The next step is the formation of the indole moiety, which is catalyzed by indole-3-glycerol phosphate synthase (IGPS; the product of trpC). This reaction comprises a ring closure of the substrate 1-(o-carboxyphenylamino)-1-deoxyribulose-5-phosphate (CdRP) into the product indole-3-glycerol phosphate (IGP). The IGPS structure has a canonical (βα)8-barrel fold with an additional N-terminal helical extension comprising two α-helices, α0 and α00, of which α0 forms a lid over the active site. In this work, we have probed the structure and mechanism of IGPS from P. aeruginosa, because it has the highest reported turnover number of all IGPS enzymes characterized to date.

The PaIGPS–rCdRP complex crystallized in space group P21212 in a large unit cell containing eight enzyme molecules per asymmetric unit. The substrate analog, rCdRP, is bound in the active site of the seven more ordered chains. rCdRP is enclosed in the active site by the helix α0 and βα-loops 1, 2, and 6. The suggested catalytic residues (Lys123, Glu172, Lys63, and Glu61) adopt similar conformations and identical interactions with the ligand rCdRP as in the SsIGPS structure. In chain B, the same conformation of rCdRP does not fit the electron density, and the ligand instead adopts a conformation where the C2' hydroxyl is shifted 2.2 Å toward the general acid Lys123. The observed movements in the C1'–C2' region in some chains are possibly coupled to the position of the guanidinium group of Arg196 on loop 6, which adopts an “inward” conformation and interacts with both the ligand's carboxylate and phosphate group in chains B, F, G, and H. Chain G lacks density for rCdRP in the active site. The helix adopts an open conformation in chain G, where—through domain swapping—it covers the active site of a symmetry-related molecule. Moreover, the disorder of these three regions reflect their innate flexibility in the apo state and suggest an induced fit mechanism of substrate binding. However, in PaIGPS, there is a phenylalanine on active-site βα-loop 6 (Phe201), 4 Å away from the anthranilate of rCdRP, whereas in EcIGPS the corresponding residue is a leucine. PaIGPS has the highest reported turnover, and from structure-guided mutagenesis we find that an active-site phenylalanine is responsible for its high activity compared with other IGPS enzymes, possibly by guiding the rate-limiting condensation step.

>[7x]MSVPTVLQKILARKAEEVAERRARVNLAEVERLARSADAPRGFANALLERAKRKEPAVIAEIKKASPSKGVLREHFVPAEIARSYEAGGAACLSVLTDVDFFQGADAYLKEARAACALPVIRKDFMIDPYQIVEARAIGADCILLIVSALDDVLMAELAATAKSVGLDVLVEVHDGTELERALKTLDTPLVGINNRNLHTFEVSLETTLDLLPEIPRDRLVVTESGILNRADVELMEVSEVYAFLVGEAFMRADDPGLELKRLFFQERGAVVLGADPDTSGHHHHHH;> XXXXXXXXXXXXXXVNLAEVERLARSADAPRGFANALLERAKRKEPAVIAEIKKASPSKGVLREHFVPAEIARSYEAGGAACLSVLTDVDFFQGADAYLKEARAACALPVIRKDFMIDPYQIVEARAIGADCILLIVSALDDVLMAELAATAKSVGLDVLVEVHDGTELERALKTLDTPLVGINNRNLHTFEVSLETTLDLLPEIPRDRLVVTESGILNRADVELMEVSEVYAFLVGEAFMRADDPGLELKRLFFQERGAVVLGADPDTSGHHHHHH> GIITCICDLNDDDGFTIQCDHC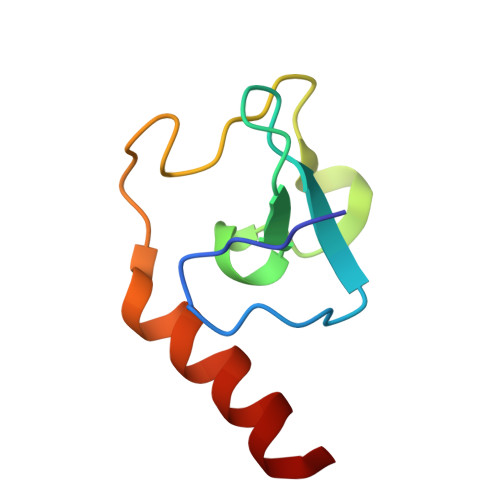NRWQHAICYGIKDIGMAPDDYLCNSCDPREVDINLARKIQQERINVK> MYSDQTYEVIKNRTLENINLDIYKGEGSFLNNMVSGNNLELSKIYLELSKMHKMAFIQDTYNQFLDKRVNEFGVYRKLGTESNGEVEFIGEKGTVINNGTIISYRDLLFVVIKDVTIGSEEGDNSPVQALEVGKKYNLPTNCEFKLVDNISGVTKITNTRSFEGGTDIETDEELKERFYKIQRNQATSGNKAHYEEWALEVDGVYNVKVYPRWDGPGTVKVLIFGKNNQAVDTETIERCQ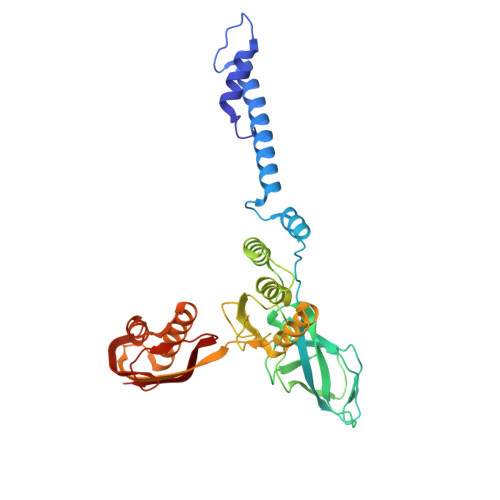QHIDEEKPIGPTITVVTPLPIEISISAVMKLEDGYTLDNVKESFLESINTYFRDIRGEIIYTKVMGILINTTGVHDLSNLLINGSTDNITINEDKIPSVTTVNFSEVENQ N~6~-methyl-N~6~-phenylpyrido[2,3-d]pyrimidine-2,4,6-triamine | C14 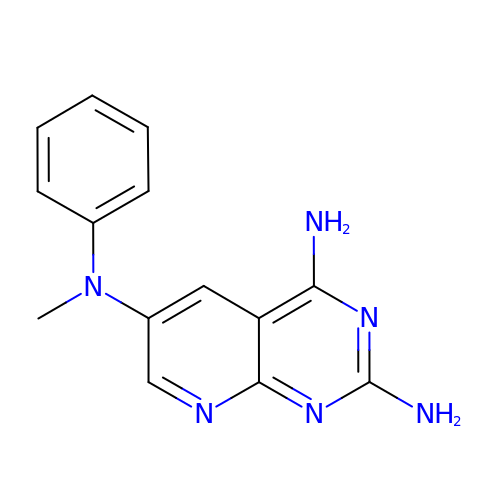H14 N6 | GPOMGDQKAATFBU-UHFFFAOYSA-N>[2x]MRVIFSEDHKLRNAKTELYGGELVPPFEAPFRAEWILAAVKEAGFDDVVAPARHGLE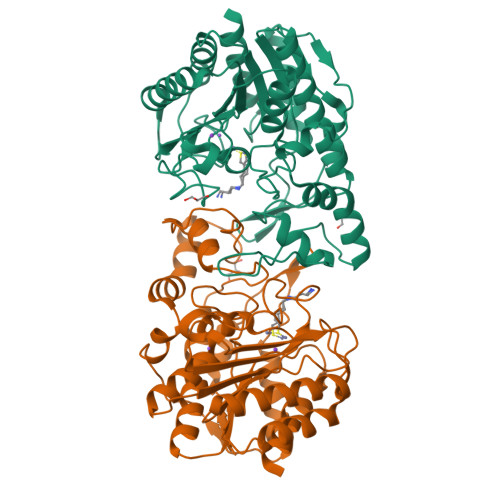TVLKVHDAGYLNFLETAWDRWKAAGYKGEAIATSFPVRRTSPRIPTDIEGQIGYYCNAAETAISPGTWEAALSSMASAIDGADLIAAGHKAAFSLCRPPGHHAGIDMFGGYCFINNAAVAAQRLLDKGAKKIAILDVDFHHGNGTQDIFYERGDVFFASLHGDPAEAFPHFLGYAEETGKGAGAGTTANYPMGRGTPYSVWGEALTDSLKRIAAFGAEAIVVSLGVDTFEQDPISFFKLTSPDYITMGRTIAASGVPLLVVMEGGYGVPEIGLNVANVLKGVAG MpPA14 (Marinomonas primoryensis PA14 domain) lectin is a domain of a 1.5-MDa adhesin responsible for a symbiotic bacterium-diatom interaction in Antarctica. Bioinformatic analyses indicated the presence of an ∼20-kDa domain near the C terminus of MpIBP that is a member of the PA14 family, which is a carbohydrate-binding lectin module widely distributed across several kingdoms of life. PA14 domains share a β-sandwich fold and the presence of two consecutive aspartate residues in a cis peptide linkage (DcisD). The DcisD motif coordinates a Ca2+ ion that is directly involved in binding polar vicinal hydroxyl groups of various carbohydrates.

We further analyzed the crystal structures of MpPA14 in complex with three pentoses, l-arabinose, ribose, and 2-deoxy-ribose, as well as inositol, which has an unusual 6-carbon saccharide ring without an endocyclic oxygen. These four carbohydrates bound MpPA14 more weakly than glucose and mannose. Crystal structures showed that MpPA14 selects the pyranose form of pentoses for binding. As pentoses have a higher percentage of furanose present in the conformational equilibria than do hexoses, selectivity for the more thermodynamically stable pyranoses might contribute to the weaker affinity of pentoses toward the lectin. For instance, despite l-arabinose existing in solution predominantly in the pyranose form at 25°C (57% α-arabinopyranose versus 30.5% β-arabinopyranose), only the α-anomer complexes MpPA14 via its 1,2-diol. The same rationale can be used to explain the even weaker affinity of ribose and its derivative 2-deoxy ribose for MpPA14 (se Fig. S5B and C in the supplemental material).

> DSTPDSLFAGLVGEYYGTNSQLNNISDFRALVDSKEADATFEAANISYGRGSSDVAKGTHLQEFLGSDASTLSTDPGDNTDGGIYLQGYVYLEAGTYNFKVTADDGYEITINGNPVATVDNNQSVYTVTHASFTISESGYQAIDMIWWDQGGDYVFQPTLSADGGSTYFVLDSAILSSTGETPYT>[3x]AITHMLRVIVESASNIPKTKFGKPDPIVSVIFKDEKKKTKKVDNELNPVWNEILEFDLRGIPLDFSSSLGIIVKDFETIGQNKLIGTATVA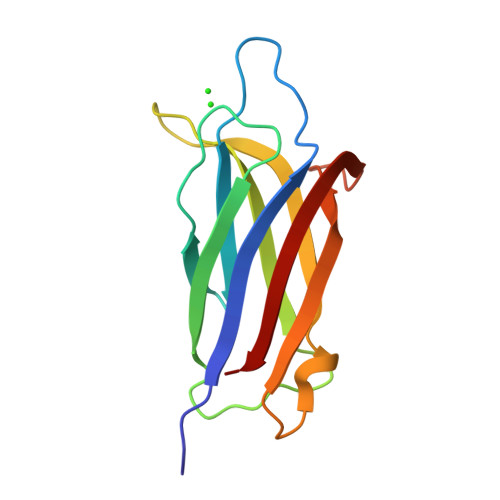LKDLTGDQSRSLPYKLISLLNEKGQDTGATIDLVIGYD>GSHMASPSNTDYPGPHSFDVSFQQSSTAKSATWTYSTELKKLYCQIAKTCPIQIKVMTPPPQGAVIRAMPVYKKAEHVTEVVKRCPNHELSREFNEGQIAPPSHLIRVEGNSHAQYVEDPITGRQSVLVPYEPPQVGTEFTTVLYNFMCNSSCVGGMNRRPILIIVTLETRDGQVLGRRCFE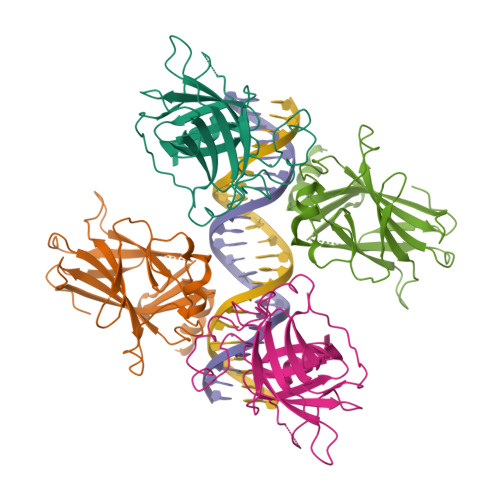ARICACPGRDRKADEDSIRKQ[2x]>[2x]MGQLIDGVWHDTWYDTKSTGGKFQRSASAFRNWLTADGAPGPTGTGGFIAEKDRYHLYVSLACPWAHRTLIMRKLKGLEPFISVSVVNPLMLENGWTFDDSFPGATGDTLYQNEFLYQLYLHADPHYSGRVTVPVLWDKKNHTIVSNESAEIIRMFNTAFDALGAKAGDYYPPALQTKIDELNGWIYDTVNNGVYKAGFATSQEAYDEAVAKVFESLARLEQILGQHRYLTGNQLTEADI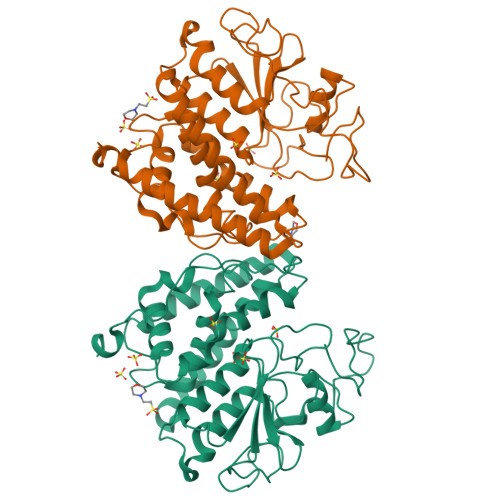RLWTTLVRFDPVYVTHFKCDKHRISDYLNLYGFLRDIYQMPGIAETVNFDHIRNHYFRSHKTINPTGIISIGPWQDLDEPHGRDVRFG>[3x]MTIFDNYEVWFVIGSQHLYGPETLRQVTQHAEHVVNALNTEAKLPCKLVLKPLGTTPDEITAICRDANYDDRCAGLVVWLHTFSPAKMWINGLTMLNKPLLQFHTQFNAALPWDSIDMDFMNLNQTAHGGREFGFIGARMRQQHAVVTGHWQDKQAHERIGSWMRQAVSKQDTRHLKVCRFGDNMREVAVTDGDKVAAQIKFGFSVNTWAVGDLVQVVNSISDGDVNALVDEYES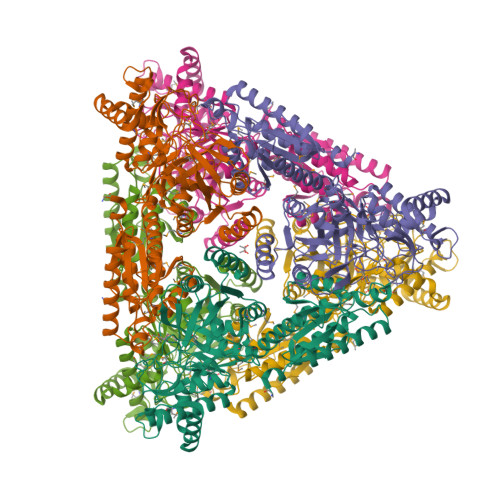CYTMTPATQIHGEKRQNVLEAARIELGMKRFLEQGGFHAFTTTFEDLHGLKQLPGLAVQRLMQQGYGFAGEGDWKTAALLRIMKVMSTGLQGGTSFMEDYTYHFEKGNDLVLGSHMLEVCPSIAVEEKPILDVQHLGIGGKDDPARLIFNTQTGPAIVASLIDLGDRYRLLVNCIDTVKTPHSLPKLPVANALWKAQPDLPTASEAWILAGGAHHTVFSHALNLNDMRQFAEMHDIEITVIDNDTRLPAFKDALRWNEVYYGFRR> SMASLKQQTGREQWASRLGFILAAMGSAVGLGNIWRFSYVTGENGGAAFLLVYLGFIALIGIPIVLAEFTIGRRAQSDAVGSFEKLAPGKPWKVAGLMGVAAGFLILSFYGVIAGWILFYLFNYITGQLWSAPAEGFGGFFEGFIANPTLPLFWQALFMIA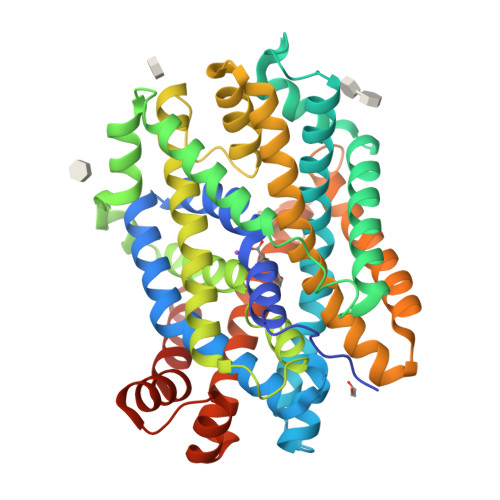TIWIVAIGVKKGIERSNKILMPLLGVLLIALAIYSLTLGGAKEGLAFLFSPDWSALKDPGVYLAAISQAFFTLSLGMGALITYGSYVSKDSRLPGAAVSVAGLDTAFAIIAGIMIFPAVFALGLSPSGGPGLVFVVLPDIFDSIRLGPIVGIAFFILLGAAALSSAVSLLEVPVAYFMRKFDWSRKQAAITLGVIITLLGIPSSLSFGVLGEVTIIPGLNIFDSVDFIASSVFLPLGGMIIALFIGWGWKTSDALAESDLTDSVWGKLWILSLRFIAPIAILIVFLSAFQIFFN> MRYSKLTMLIPCALLLSACTTVTPAYKDNGTRSGPCVEGGPDNVAQQFYDYRILHRSNDITALRPYLSDKLATLLSDASRDNNHRELLTNDPFSSRTTLPDSAHVASASTIPNRDARNIPLRVDLKQGDQGWQ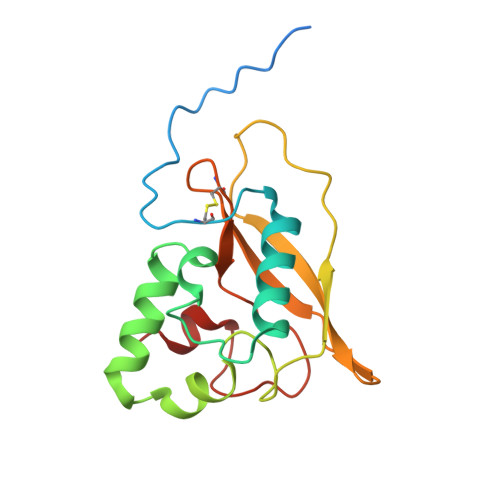DEVLMIQEGQCWVIDDVRYLGGSVHATAGTLRQSIENR>[5x]MKITVVDLGNINVKYVGENKGRFSSKITNDYQSYEEGFQRVEYNGIKTYIGVGELSREFNKADRDYMAQLLYSLAKANTADTKEINLTLLLPIIQMKNKTRLIETLKGENFKFKFNGIDREIKINDLMVLPEGYASYYSLDIENKKGDVCILDLGSRTINICVLENAKIVKTNTIKLGSFDFYSKIKSLENAKGEDYIEEDIQRLIDNGLIKVDSKQYIEFLSDILNAVKPYVN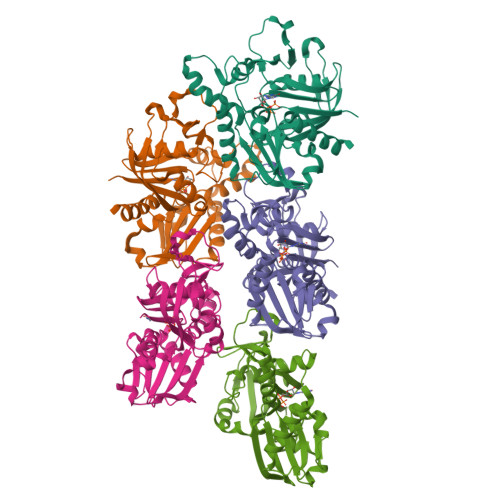LKTYNTIFTGGTSLMLKEYIEKLPLNKFKVHPNALTSNVDGAMEASKKVWN>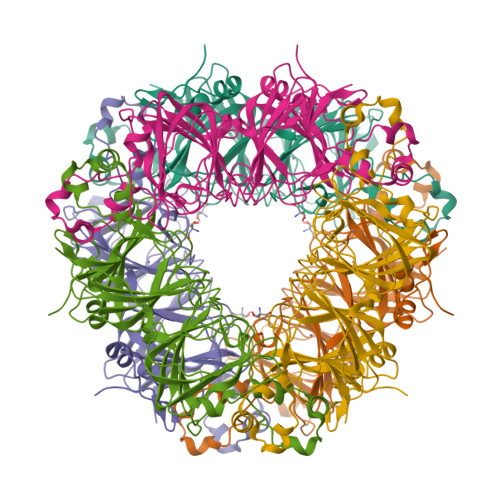 MKKQNDIPQPIRGDKGATVKIPRNIERDRQNPDMLVPPETDHGTVSNMKFSFSDTHNRLEKGGYAREVTVRELPISENLASVNMRLKPGAIAELHWHKEAEWAYMIYGSARVTIVDEKGRSFIDDVGEGDLWYFPSGLPHSIQALEEGAEFLLVFDDGSFSENSTFQLTDWLAHTPKEVIAANFGVTKEEISNLPGKEKYIFENQLPGSLKDDIVEGPNGEVPYPFTYRLLEQEPIESEGGKVYIADSTNFKVSKTIASALVTVEPGAMRELHWHPNTHEWQYYISGKARMTVFASDGHARTFNYQAGDVGYVPFAMGHYVENIGDEPLVFLEIFKDDHYADVSLNQWLAMLPETFVQAHLDLGKDFTDVLSKEKHPVVKKKCSK> NKVIQLQKIFQSSTKPLWWRHPRSALYLYPFYAIFAV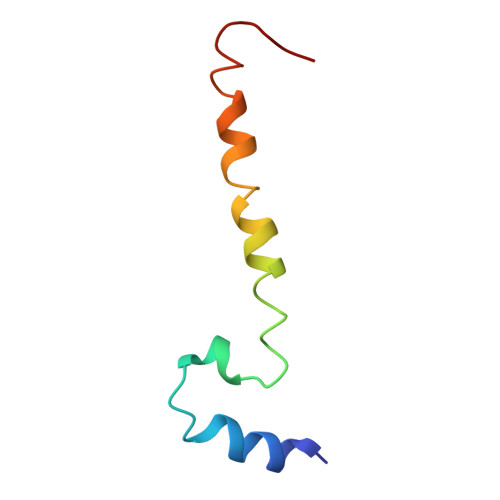AVVTPLLYIPNAIRGIKA>GPHMADDVVITARN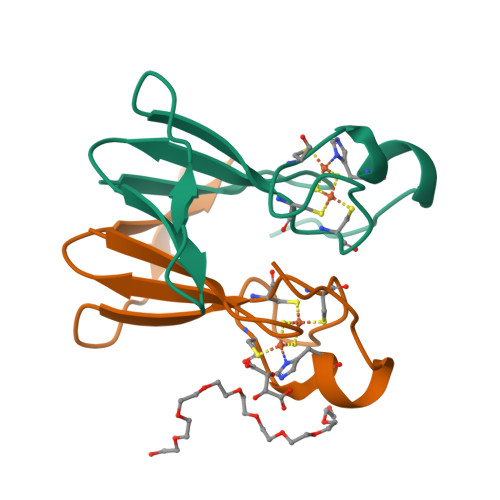NGPYHIKGSFRIVTQGGRELPVEQGQAWLCRCGHSLNKPFCDGSHKRVEFDSNLD[2x]6-hexyl-5-phenyl-pyrimidine-2,4-diamine | C16 H22 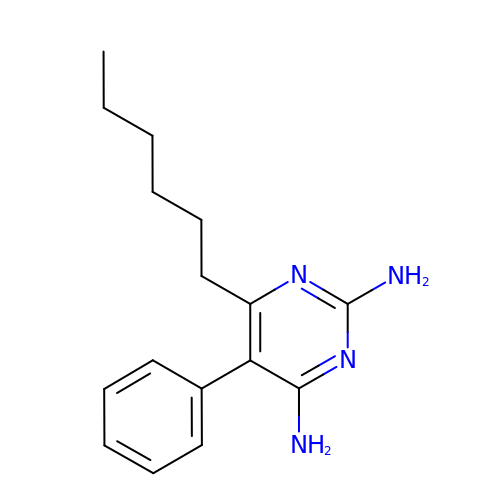N4 | DBCDYKFZHWOABJ-UHFFFAOYSA-N>[2x]MKTIIINGVQFNTDEDTTILKFARDNNIDISALCFLNNCNNDINKCEICTVEVEGTGLVTACDTLIEDGMIINTNSDAVNEKIKSRISQLLDIHEFKCGPCNRRENCEFLKLVIKYKARASKPFLPKDKTEYVDERSKSLTVDRTKCLLCGRCVNACGKNTETYAMKFLNKNGKTIIGAEDEKCFDDTNCLLCGQCIIACPVAALSEKSHMDRVKNALNAPEKHVIVAMAPSVRASIGELFNMGFGVDVTGKIYTALRQLGFDKIFDINFGADMTIMEEATELVQRIENNGPFPMFTSCCPGWVRQAENYYPELLNNLSSAKSPQQIFGTASKTYYPSISGLDPKNVFTVTVMPCTSKKFEADRPQMEKDGLRDIDAVITTRELAKMIKDAKIPFAKLEDSEADPAMGEYSGAGAIFGATGGVMEAALRSAKDFAENAELEDIEYKQVRGLNGIKEAEVEINNNKYNVAVINGASNLFKFMKSGMINEKQYHFIEVMACHGGCVNGGGQPHVNPKDLEKVDIKKVRASVLYNQDEHLSKRKSHENTALVKMYQNYFGKPGEGRAHEILHFKYKKSAWSHPQFEK

pmcHydrogenases are metalloenzymes that catalyze the interconversion between protons (H+), electrons (e−) and hydrogen (H2). Among them, [FeFe]‐hydrogenases exhibit the highest activity for both H2 production and oxidation. Their catalytic cofactor, termed H‐cluster, consists of a [4Fe4S] sub‐cluster ([4Fe]H) and a diiron moiety ([2Fe]H) bridged through a cysteine residue. The amine base is connected to the protein surface through a conserved proton transfer pathway (PTP) for rapid H+ shuttling.

Two crystals of 1.39 Å and 1.5 Å, termed CpI‐CN−‐1 and CpI‐CN−‐2 in the following, were analyzed in depth. The refined occupancies indicate that the OCS is fully occupied by an extrinsic ligand in CN−‐treated CpI, whereas only 71 to 93 % of the OCS of CO‐treated crystals hold an extrinsic ligand. In the two structures CpI‐CN−‐1 and CpI‐CN−‐2, the distances between C299 and the amine group of the [2Fe]H subcluster are larger than those in Hox in both chains A and B. The side chain of E279 is slightly twisted and consequently closer to S319, whereas the distance between E279 and Wat1 increases in several cases. Wat1 and Wat2 are also shifted; in all cases, Wat1 lies about 0.6 to 1 Å closer to the surface. Consequently, the H‐bond length between C299 and Wat1 is longer than in the Hox state. The electron densities of E282 revealed varying conformations. In chain B of CpI‐CN−‐2, E282 is twisted towards the surface and out of H‐bond length to S319. In chain B of CpI‐CN−‐1 and chain A of CpI‐CN−‐2, this residue was modeled in two conformations. The structural changes in PTP elements observed in our CN−‐treated crystals have been proposed to be necessary for efficient catalytic H+ transport, but they have never been observed structurally in wild type [FeFe]‐hydrogenases.>[4x]MLESKLKAPVFTATTQGDHYGEFVLEPLERGFGVTLGNPLRRILLSSIPGTAVTSVYIEDVLHEFSTIPGVKEDVVEIILNLKELVVRFLDPKMASTTLILRAEGPKEVRAGDFTPSADVEIMNPDLHIATLEEGGKLYMEVRVDRGVGYVPAERHGIKDRINAIPVDAIFSPVRRVAFQVEDTRLGQRTDLDKLTLRIWTDGSVTPLEALNQAVAILKEHLNYFANPEASLLPTPEVSKGEKRESAEEDLDLPLEELGLSTRVLHSLKEEGIESVRALLALNLKDLRNIPGIGERSLEEIRQALAKKGFTLKE;>[2x]MEIKRFGRIREVIPLPPLTEIQVESYKKALQADVPPEKRENVGIQAAFKETFPIEEGDKGKGGLVLDFLEYRIGDPPFSQDECREKDLTYQAPLYARLQLIHKDTGLIKEDEVFLGHLPLMTEDGSFIINGADRVIVSQIHRSPGVYFTPDPARPGRYIASIIPLPKRGPWIDLEVEASGVVTMKVNKRKFPLVLLLRVLGYDQETLVRELSAYGDLVQGLLDEAVLAMRPEEAMVRLFTLLRPGDPPKKDKALAYLFGLLADPKRYDLGEAGRYKAEEKLGVGLSGRTLVRFEDGEFKDEVFLPTLRYLFALTAGVPGHEVDDIDHLGNRRIRTVGELMADQFRVGLARLARGVRERMVMGSPDTLTPAKLVNSRPLEAALREFFSRSQLSQFKDETNPLSSLRHKRRISALGPGGLTRERAGFDVRDVHRTHYGRICPVETPEGANIGLITSLAAYARVDALGFIRTPYRRVKNGVVTEEVVYMTASEEDRYTIAQANTPLEGDRIATDRVVARRRGEPVIVAPEEVEFMDVSPKQVFSLNTNLIPFLEHDDANRALMGSNMQTQAVPLIRAQAPVVMTGLEERVVRDSLAALYAEEDGEVVKVDGTRIAVRYEDGRLVEHPLRRYARSNQGTAFDQRPRVRVGQRVKKGDLLADGPASEEGFLALGQNVLVAIMPFDGYNFEDAIVISEELLKRDFYTSIHIERYEIEARDTKLGPERITRDIPHLSEAALRDLDEEGIVRIGAEVKPGDILVGRTSFKGEQEPSPEERLLRSIFGEKARDVKDTSLRVPPGEGGIVVGRLRLRRGDPGVELKPGVREVVRVFVAQKRKLQVGDKLANRHGNKGVVAKILPVEDMPHLPDGTPVDVILNPLGVPSRMNLGQILETHLGLAGYFLGQRYISPVFDGATEPEIKELLAEAFNLYFGKRQGEGFGVDKREKEVLARAEKLGLVSPGKSPEEQLKELFDLGKVVLYDGRTGEPFEGPIVVGQMFIMKLYHMVEDKMHARSTGPYSLITQQPLGGKAQFGGQRFGEMEVWALEAYGAAHTLQEMLTIKSDDIEGRNAAYQAIIKGEDVPEPSVPESFRVLVKELQALALDVQTLDEKDNPVDIFEGLASKR;>MKKEVRKVRIALASPEKIRSWSYGEVEKPETINYRTLKPERDGLFDERIFGPIKDYECACGKYKRQRFEGKVCERCGVEVTRSIVRRYRMGHIELATPAAHIWFVKDVPSKIGTLLDLSATELEQVLYFNKYIVLDPKGAVLDGVPVEKRQLLTDEEYRELRYGKQETYPLPAGVDALVKDGEEVVKGQELAPGVVSRMDGVALYRFPRRVRVDYLRKERAALRIPLSAWVEKEAYRPGEVLAELSEPYLFRAEESGVVELKDLAEGHLIYLRQEEEVVARYFLPAGMTPLVVEGEIVEVGQPLAEGKGLLRLPRHMTAKEVEAEEEGDSVHLTLFLEWTEPKDYKVAPHMNVIVPEGAKVQAGEKIVAAIDPEEEVIAEAEGVVHLHEPASILVVKARVYPFEDDVEVTTGDRVAPGDVLADGGKVKSEIYGRVEVDLVRNVVRVVESYDIDARMGAEAIQELLKELDLEKLERELLEEMK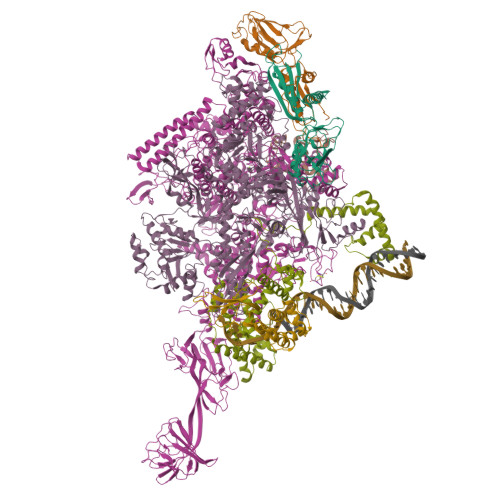HPSRARRAKARKRLEVVRAFLDSGNRPEWMILEAVPVLPPDLRPMVQVDGGRFATSDLNDLYRRLINRNNRLKKLLAQGAPEIIIRNEKRMLQEAVDAVIDNGRRGSPVTNPGSERPLRSLTDILSGKQGRFRQNLLGKRVDYSGRSVIVVGPQLKLHQCGLPKRMALELFKPFLLKKMEEKAFAPNVKAARRMLERQRDIKDEVWDALEEVIHGKVVLLNRAPTLHRLGIQAFQPVLVEGQSIQLHPLVCEAFNADFDGDQMAVHVPLSSFAQAEARIQMLSAHNLLSPASGEPLAKPSRDIILGLYYITQVRKEKKGAGMAFATPEEALAAYERGEVALNAPIVVAGRETSVGRLKFVFANPDEALLAVAHGLLDLQDVVTVRYLGRRLETSPGRILFARIVGEAVGDEKVAQELIQMDVPQEKNSLKDLVYQAFLRLGMEKTARLLDALKYYGFTLSTTSGITIGIDDAVIPEEKQRYLEEADRKLRQIEQAYEMGFLTDRERYDQVIQLWTETTEKVTQAVFKNFEENYPFNPLYVMAQSGARGNPQQIRQLCGMRGLMQKPSGETFEVPVRSSFREGLTVLEYFISSHGARKGGADTALRTADSGYLTRKLVDVAHEIVVREADCGTTNYISVPLFQMDEVTRTLRLRKRSDIESGLYGRVLAREVEALGRRLEEGRYLSLEDVHFLIKAAEAGEVREVPVRSPLTCQTRYGVCQKCYGYDLSMARPVSIGEAVGVVAAESIGEPGTQLTMRTFHTGGVAVGTDITQGLPRVIELFEARRPKAKAVISEIDGVVRIEEGEDRLSVFVESEGFSKEYKLPKDARLLVKDGDYVEAGQPLTRGAIDPHQLLEAKGPEAVERYLVDEIQKVYRAQGVKLHDKHIEIVVRQMLKYVEVTDPGDSRLLEGQVLEKWDVEALNERLIAEGKVPVAWKPLLMGVTKSALSTKSWLSAASFQNTTHVLTEAAIAGKKDELIGLKENVILGRLIPAGTGSDFVRFTQVVDQRTLKAIEEARKEAVEAKEKEAPRRPVRREQPGKGL[2x];>[2x]MAEPGIDKLFGMVDSKYRLTVVVAKRAQQLLRHRFKNTVLEPEERPKMRTLEGLYDDPNAVTWAMKELLTGRLFFGENLVPEDRLQKEMERLYPTEEEA;>[2x]TSDPVRQYLHEIGQVPLLTLEEEIDLARKVEEGMEAIKKLSEATGLDQELIREVVRAKILGTARIQKIPGLKEKPDPKTVEEVDGKLKSLPKELKRYLHIAREGEAARQHLIEANLRLVVSIAKKYTGRGLSFLDLIQEGNQGLIRAVEKFEYKRRFKFSTYATWWIRQAINRAIADQARTIRIPVHMVETINKLSRTARQLQQELGREPSYEEIAEAMGPGWDAKRVEETLKIAQEPVSLETPIGDEKDSFYGDFIPDENLPSPVEAAAQSLLSEELEKALSKLSEREAMVLKLRKGLIDGREHTLEEVGAYFGVTRERIRQIENKALRKLKYHESRTRKLRDFLE;>MKEFRPGDKVVLPPYGVGVVAGIAQRSVSGVSRAYYQVDFPGSRSKAYVPVEAPHSVGLRKALAPEEVPVILDLLKNGRMPLPKQWAARHRKTSEILADGNPYRIAQMAGQLRAWEVERGLPDLDRQALRRAIHLLAEEVAQSLEITVQEAKRLFEEAWGEELN[2x]>AQLVDSMPSASTGSVVVTDDLNYWGGRRIKSKDGATTEPVFEPATGRVLCQMVPCGAEEVDQAVQSAQAAYLKWSKMAGIERSRVMLEAARIIRERRDNIAKLEVINNGKTITEAEYDIDAAWQCIEYYAGLAPTLSGQHIQLPGGAFAYTRREPLGVCAGILAWNYPFMIAAWKCAPALACGNAVVFKPSPMTPVTGVILAEIFHEAGVPVGLVNVVQGGAETGSLLCHHPNVAKVSFTGSVPTGKKVMEMSAKTVKHVTLELG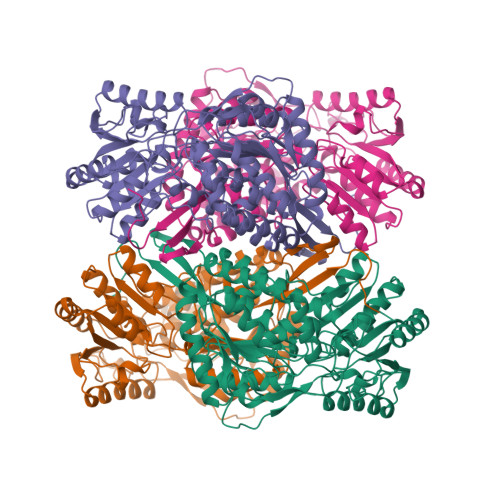GKSPLLIFKDCELENAVRGALMANFLTQGQVCTNGTRVFVQREIMPQFLEEVVKRTKAIVVGDPLLTETRMGGLISKPQLDKVLGFVAQAKKEGARVLCGGEPLTPSDPKLKNGYFMSPCVLDNCRDDMTCVKEEIFGPVMSVLPFDTEEEVLQRANNTTFGLASGVFTRDISRAHRVAANLEAGTCYINTYSISPVEVPFGGYKMSGFGRENGQATVDYYSQLKTVIVEMGDVDSLF[4x]> 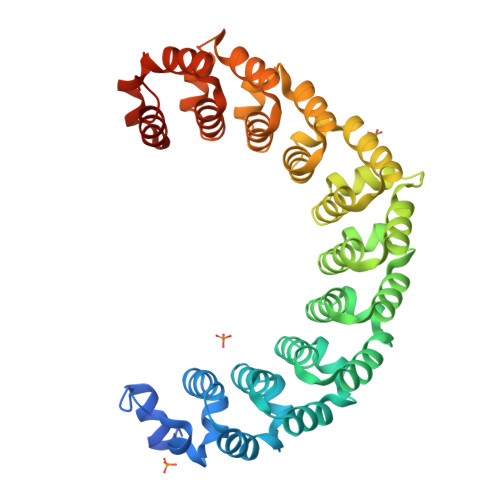MGSSHHHHHHSQDLEVLFQGPHMGRSRLLEDFRNNRYPNLQLREIAGHIMEFSQDQHGSRFIQLKLERATPAERQLVFNEILQAAYQLMVDVFGNYVIQKFFEFGSLEQKLALAERIRGHVLSLALQMYGCRVIQKALEFIPSDQQNEMVRELHQHTEQLVQDQYGNYVIQHVLEHGRPEDKSKIVAEIRGNVLVLSQHKFASNVVEKCVTHASRTERAVLIDEVCTMNDGPHSALYTMMKDQYANYVVQKMIDVAEPGQRKIVMHELHQHTEQLVQDQYGNYVIQHVLEHGRPEDKSKIVAEIRGNVLVLSQHKFASNVVEKCVTHASRTERAVLIDEVCTMNDGPHSALYTMMKDQYANYVVQKMIDVAEPGQRKIVMHKIRPHIATLRKYTYGKHILAKLEKYYMKNGVDLG>[2x]AALPDSVDWREKGCVTEVKYQGSCGASWAFSAVGALEAQLKLKTGKLVSLSAQNLVDCSTEKYGNKGCNGGFMTTAFQYIIDNKGIDSDASYPYKAMDQKCQYDSKYRAATCSKYT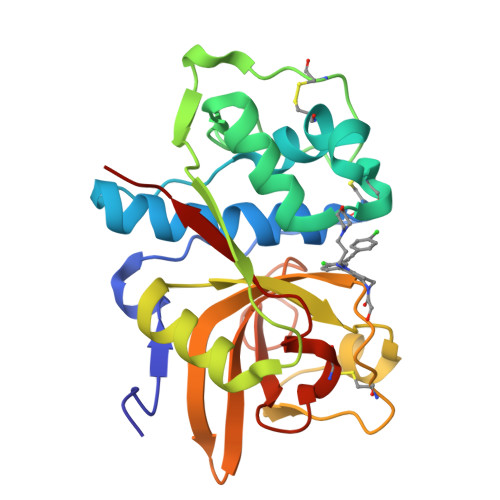ELPYGREDVLKEAVANKGPVSVGVDARHPSFFLYRSGVYYEPSCTQNVNHGVLVVGYGDLNGKEYWLVKNSWGHNFGEEGYIRMARNKGNHCGIASFPSYPEILQG> QDADKLPHTKVTLVAPPQVHPHEQATKSGPKVVEFTMTIEEKKMVIDDKGTTLQA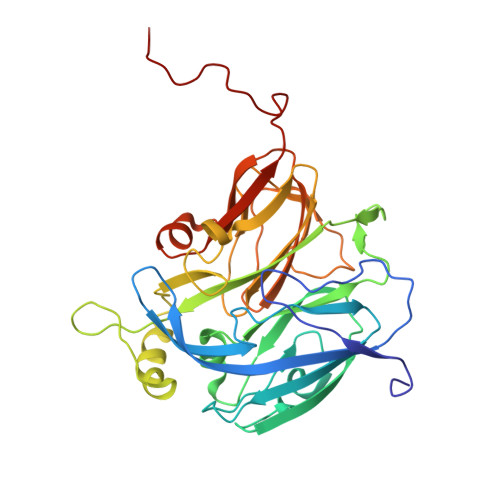MTFNGSMPGPTLVVHEGDYVQLTLVNPATNAMPHNVDFHGATGALGGAKLTNVNPGEQATLRFKADRSGTFVYHCAPEGMVPWHVVSGMSGTLMVLPRDGLKDPQGKPLHYDRAYTIGEFDLYIPKGPDGKYKDYATLAESYGDTVQVMRTLTPSHIVFNGKVGALTGANALTAKVGETVLLIHSQANRDTRPHLIGGHGDWVWETGKFANPPQRDLETWFIRGGSAGAALYTFKQPGVYAYLNHNLIEAFELGAAGHIKVEGKWNDDLMKQIKAPAPIPR>[2x]MGFFDRLKAGLAKTRERLLKAIPWGGNLEEVLEELEMALLAADVGLSATEEILQEVRASGRKDLKEAVKEKLVGMLEPD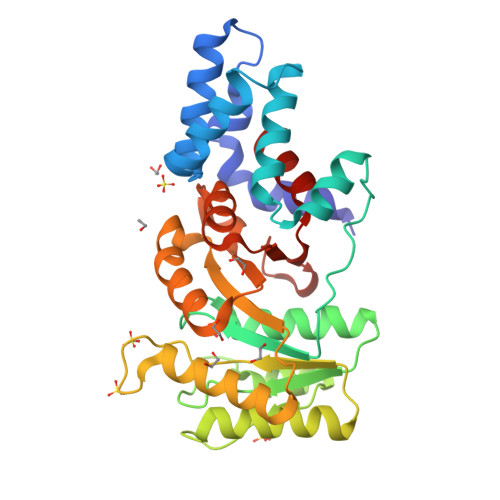ERRATLRKLGFNPQKPKPVEPKGRVVLVVGVNGVGKTTTIAKLGRYYQNLGKKVMFCAGDTFRAAGGTQLSEWGKRLSIPVIQGPEGTDPAALAYDAVQAMKARGYDLLFVDTAGRLHTKHNLMEELKKVKRAIAKADPEEPKEVWLVLDAVTGQNGLEQAKKFHEAVGLTGVIVTKLDGTAKGGVLIPIVRTLKVPIKFVGVGEGPDDLQPFDPEAFVEALLED>MNSSSFPYFISPEQAMRERSELARKGIARAKSVVALAYAGGVLFVAENPSRSLQKISELYDRVGFAAAGKFNEFDNLRRGGIQFADTRGYAYDRRDVTGRQLANVYAQTLGTIFTEQAKPYEVELCVAEVAHYGETKRPELYRITYDGSIADEPHFVVMGGTTEPIANALKESYAENASLTDALRIAVAALRAGSADTSGGDQPTLGVASLEVAVLDANRPRRAFRRITGSALQALLVDQESPQSDGESSG[14x];>[14x]TTIVALKYPGGVVMAGDRRSTQGNMISGRDVRKVYITDDYTATGIAGTAAVAVEFARLYAVELEHYEKLEGVPLTFAGKINRLAIMVRGNLAAAMQGLLALPLLAGYDIHASDPQ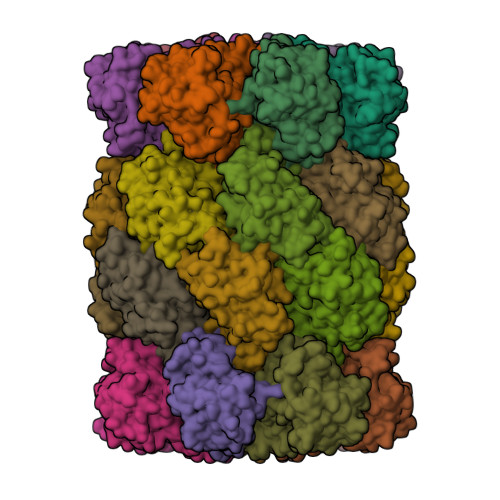SAGRIVSFDAAGGWNIEEEGYQAVGSGSLFAKSSMKKLYSQVTDGDSGLRVAVEALYDAADDDSATGGPDLVRGIFPTAVIIDADGAVDVPESRIAELARAIIESRSGADTFGSDGGEKHHHHHH2-{(2E,4aR,7aR)-7a-[4-(3-cyanophenyl)thiophen-2-yl]-2-imino-3-methyl-4-oxooctahydro-6H-pyrrolo[3,4-d]pyrimidin-6-yl}pyridine-3-carbonitrile | C24 H19 N7 O S | 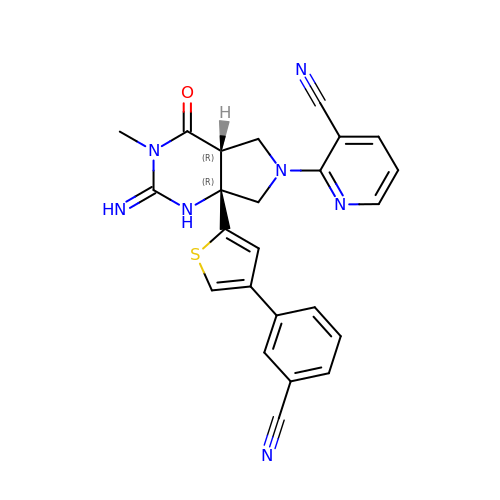LWVMTILRDSZVMA-CYFREDJKSA-N> AWPKVQPEVNIGVVGHVDHGKTTLVQAITGIWTSKHSEETIKLGYAETNIGVCESCKKPEAYVTEPSCKSCGSDDEPKFLRRISFIDAPGHEVLMATMLSGAALMDGAILVVAANEPFPQPQTREHFVALGIIGVKNLIIVQNKVDVVSKEEALSQYRQIKQFTKGTWAENVPIIPVSALHKINIDSLIEGIEEYIKTPYRDLSQKPVMLVIRSFDVNKPGTQFNELKGGVIGGSIIQGLFKVDQEIKVLPGLRVEKQGKVS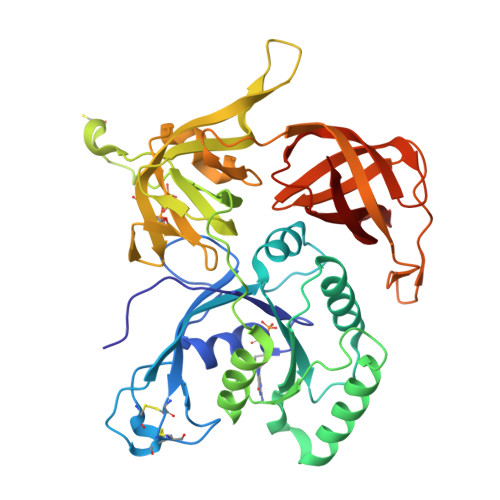YEPIFTKISSIRFGDEEFKEAKPGGLVAIGTYLDPSLTKADNLLGSIITLADAEVPVLWNIRIKYNLLERVVGAKEMLKVDPIRAKETLMLSVGSSTTLGIVTSVKKDEIEVELRRPVAVWSNNIRTVISRQIAGRWRMIGWGLVEI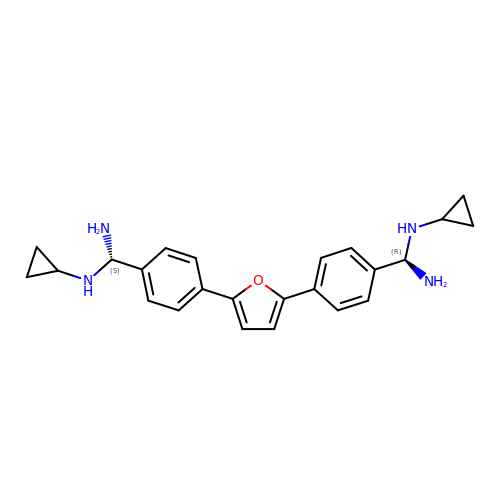2,5-BIS{[4-(N-CYCLOPROPYLDIAMINOMETHYL)PHENYL]}FURAN | C24 H28 N4 O | YKBBTHHMEIPZMC-PSWAGMNNSA-N(2~{R},4~{R})-2,5,5-trimethyl-1,3-thiazolidine-2,4-dicarboxylic acid | 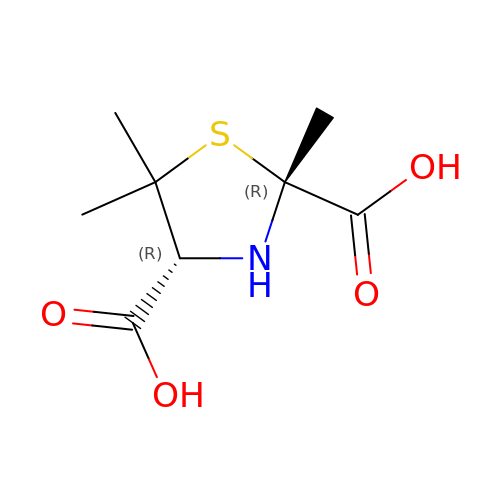C8 H13 N O4 S | VYZKCSMVPAWSBH-SPGJFGJESA-N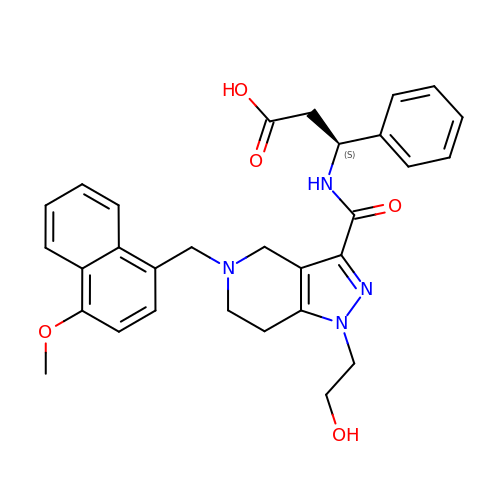(3~{S})-3-[[1-(2-hydroxyethyl)-5-[(4-methoxynaphthalen-1-yl)methyl]-6,7-dihydro-4~{H}-pyrazolo[4,3-c]pyridin-3-yl]carbonylamino]-3-phenyl-propanoic acid | C30 H32 N4 O5 | FEINFPMXJVPOSJ-VWLOTQADSA-N> MKSLIFTLSLLALTGCTITRQAQVSEASPISGIVRLTYNQPLFFTSRTDDYVSHGTATRE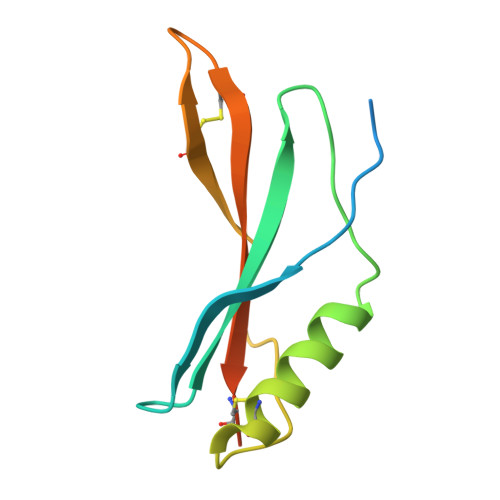CQQMGYADAVSFGQPVGTCSIYAGSLCLNTRFTLSWQCRGVAVPQIMPLYY N-[(5R,6R,7R,8S)-6,7-DIHYDROXY-5-(HYDROXYMETHYL)-2-(2-PHENYLETHYL)-5,6,7,8-TETRAHYDROIMIDAZO[1,2-A]PYRIDIN-8-YL]-3-SULFANYLPROPANAMIDE | C19 H25 N3 O4 S | 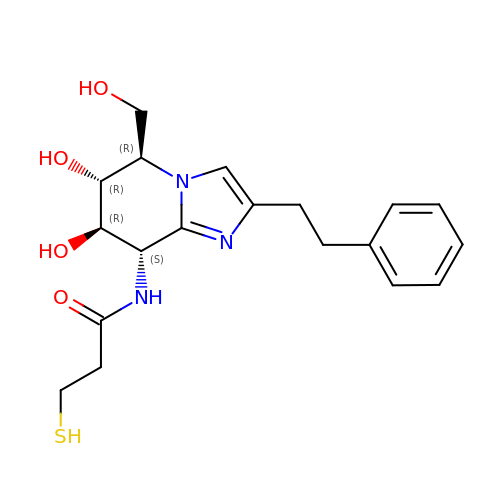ZEEDRHPJCAOZKV-VDHUWJSZSA-N>MHHHHHHASGLVPRGSHMTRTTALKVLAGKKLTDLDPDEWAKAQASAERILVDVGTGDARTAYRQAIAHPEWLVVGVDPAWQRMTETAVRAARKPAKGGAPNLVLVSSA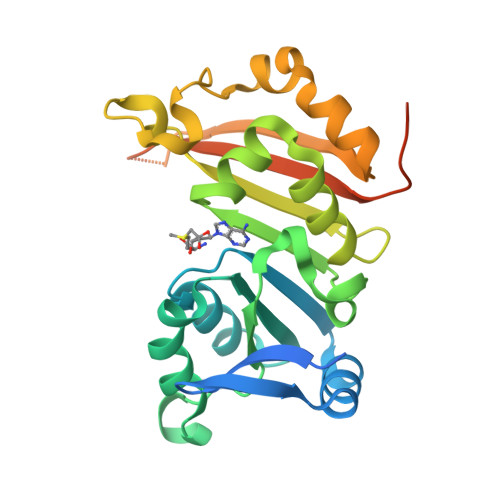IETVPAALHGVADEVMVLMPWGKLLRGVVLGEADVLSGLRAVAKPGAPLEISIGTSIWREPIPLEIRDLPELTPETVVSTGLTDRLAALGWQVADVRLVPHTDLDTISSSAARRLGSGATETVLHLRAVAVDPRDPVGTQHPAAESAQDTPEEPQRDV[2x]>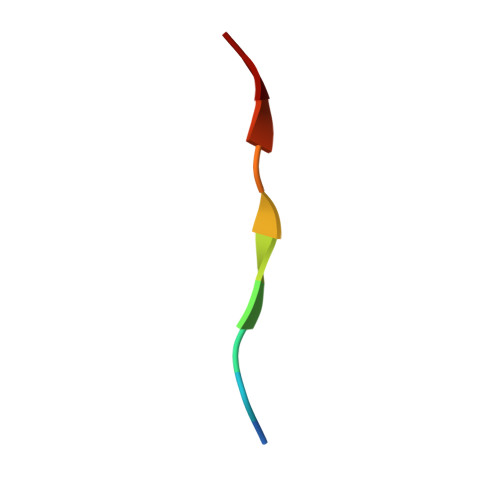 QPELYLLNTM Evidence accumulated over the past two decades has identified titin as a main coordinator of cardiac muscle homeostasis, and its dysfunction through genetic mutation as an important factor in cardiomyopathy. For this, we examined the unique mSNP T2850I in the I-band domain of titin I10, as a paradigm of an alteration in a general component of the titin chain. Domain I10 does not support specific interactions or have any known specialized roles, so it does not constitute an a priori sensitive locus of the chain. In previous studies, we have shown that the T2580I mSNP destabilizes the affected immunoglobulin (Ig) domain in titin, I10, and speculated that this instability increases the vulnerability of titin to proteolysis in situ potentially leading to myocardial damage.

Residue T2850 is located at the C-terminal loop region of the Ig fold. To study whether this region is involved in interactions with the next Ig domain packed serially along the chain and, thus, whether the T2850I exchange influences the Ig-tandem architecture of titin, we determined the crystal structure of I9–I11 (comprising I10 in its poly-domain context) to 1.53 Å resolution. Three molecular copies were obtained in two space groups that agreed in showing I9–I11 in an extended conformation. Such extended arrangements are common in titin Ig-tandems. In I9–I11, the component domains follow a regular arrangement, where domains display relative torsion angles of 45°–68° and are connected by short, two-residue sequences (TL and PI, respectively). In each Ig-pair, the domain interface is consistently formed by the A'B β-turn of the N-terminal domain slotting between the BC and FG loops of the C-terminal domain. Here, domains interact directly through a limited number of contacts (section S2). Both I9–I10 and I10–I11 interfaces consist of a central hydrophobic residue contributed by the linker sequence (TL; PI), flanked by two polar interactions between loop residues from the neighbouring domains (inset). Residue T2850 is buried within the I10–I11 interface (burial fraction of side chain is 0.79 as calculated with FoldX). Here, T2850 preserves its intradomain hydrogen bonds (to T2897 and E2849) observed in the isolated I10 structure and, in addition, hydrogen bonds with S2952 from the BC loop of I11. This suggests that the exchange of the T2850 residue will cause a local alteration of the conformational dynamics of the titin chain.

> GAMVKIIKKPKDVTALENATVAFEVSVSHDTVPVKWFHKSVEIKPSDKHRLVSERKVHKLMLQNISPSDAGEYTAVVGQLECKAKLFVETLHITKTMKNIEVPETKTASFECEVSHFNVPSMWLKNGVEIEMSEKFKIVVQGKLHQLIIMNTSTEDSAEYTFVCGNDQVSATLTVTPIMITSMLKDINAEEKDTITFEVTVNYEGISYKWLKNGVEIKSTDKCQMRTKKLTHSLNIRNVHFGDAADYTFVAGKATSTATLYVVEA>[2x]FQASPSQSLYREIHQLISFKDVLPDKNLLPDWSSNKNPCTFDGVTCRDDKVTSIDLSSKPLNVGFSAVSSSLLSLTGLESLFLSNSHINGSVSGFKCSASLTSLDLSRNSLSGPVTTLTSLGSCSGLKFLNVSSNTLDFPGKVSGGLKLNSLEVLDLSANSISGANVVGWVLSDGCGELKHLAISGNKISGDVDVSRCVNLEFLDVSSNNFSTGIPFLGDCSALQHLDISGNKLSGDFSRAISTCTELKLLNISSNQFVGPIPPLPLKSLQYLSLAENKFTGEIPDFLSGACDTLTGLDLSGNHFYGAVPPFFGSCSLLESLALSSNNFSGELPMDTLLKMRG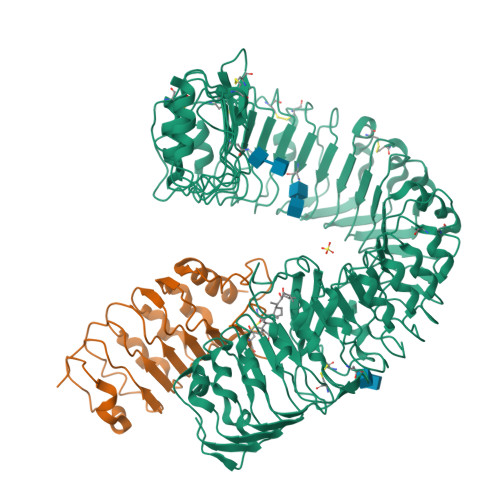LKVLDLSFNEFSGELPESLTNLSASLLTLDLSSNNFSGPILPNLCQNPKNTLQELYLQNNGFTGKIPPTLSNCSELVSLHLSFNYLSGTIPSSLGSLSKLRDLKLWLNMLEGEIPQELMYVKTLETLILDFNDLTGEIPSGLSNCTNLNWISLSNNRLTGEIPKWIGRLENLAILKLSNNSFSGNIPAELGDCRSLIWLDLNTNLFNGTIPAAMFKQSGKIAANFIAGKRYVYIKNDGMKKECHGAGNLLEFQGIRSEQLNRLSTRNPCNITSRVYGGHTSPTFDNNGSMMFLDMSYNMLSGYIPKEIGSMPYLFILNLGHNDISGSIPDEVGDLRGLNILDLSSNKLDGRIPQAMSALTMLTEIDLSNNNLSGPIPEMGQFETFPPAKFLNNPGLCGYPLPRCDPSNADGYAHHQRSHHHHHH;>[2x]NAEGDALSALKNSLADPNKVLQSWDATLVTPCTWFHVTCNSDNSVTRVDLGNANLSGQLVMQLGQLPNLQYLELYSNNITGTIPEQLGNLTELVSLDLYLNNLSGPIPSTLGRLKKLRFLRLNNNSLSGEIPRSLTAVLTLQVLDLSNNPLTGDIPVNGSFSLFTPISFANTKLTPLPASPPPPISPTPPSPAGSHHHHHH> MTTYLEFIQQNEERDGVRFSWNVWPSSRLEATRMVVPV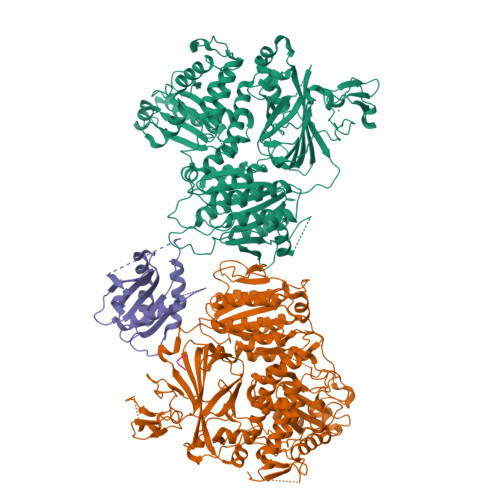AALFTPLKERPDLPPIQYEPVLCSRTTCRAVLNPLCQVDYRAKLWACNFCYQRNQFPPSYAGISELNQPAELLPQFSSIEYVVLRGPQMPLIFLYVVDTCMEDEDLQALKESMQMSLSLLPPTALVGLITFGRMVQVHELGCEGISKSYVFRGTKDLSAKQLQEMLGLSKVPLTQATRGPQVQQPPPSNRFLQPVQKIDMNLTDLLGELQRDPWPVPQGKRPLRSSGVALSIAVGLLECTFPNTGARIMMFIGGPATQGPGMVVGDELKTPIRSWHDIDKDNAKYVKKGTKHFEALANRAATTGHVIDIYACALDQTGLLEMKCCPNLTGGYMVMGDSFNTSLFKQTFQRVFTKDMHGQFKMGFGGTLEIKTSREIKISGAIGPCVSLNSKGPCVSENEIGTGGTCQWKICGLSPTTTLAIYFEVVNQHNAPIPQGGRGAIQFVTQYQHSSGQRRIRVTTIARNWADAQTQIQNIAASFDQEAAAILMARLAIYRAETEEGPDVLRWLDRQLIRLCQKFGEYHKDDPSSFRFSETFSLYPQFMFHLRRSSFLQVFNNSPDESSYYRHHFMRQDLTQSLIMIQPILYAYSFSGPPEPVLLDSSSILADRILLMDTFFQILIYHGETIAQWRKSGYQDMPEYENFRHLLQAPVDDAQEILHSRFPMPRYIDTEHGGSQARFLLSKVNPSQTHNNMYAWGQESGAPILTDDVSLQVFMDHLKKLAVSSA;> EGLRVVNLLQERNMLPSTPLKPPVPNLHEDIQKLNCNPELFRCTLTSIPQTQALLNKAKLPLGLLLHPFKDLVQLPVVTSSTIVRCRSCRTYINPFVSFLDQRRWKCNLCYRVNDVPEEFLYNPLTRVYGEPHRRPEVQNATIEFMAPSEYMLRPPQPPVYLFVFDVSHNAVETGYLNSVCQSLLDNLDLLPGNTRTKIGFITFDSTIHFYGLQESLSQPQMLIVSDIEDVFIPMPENLLVNLNESKELVQDLLKTLPQMFTKTLETQSALGPALQAAFKLMSPTGGRMSVFQTQLPTLGVGALKPREEPNHRSSAKDIHMTPSTDFYKKLALDCSGQQVAVDLFLLSGQYSDLASLGCISRYSAGSVYYYPSYHHQHNPVQVQKLQKELQRYLTRKIGFEAVMRIRCTKGLSIHTFHGNFFVRSTDLLSLPNVNPDAGYAVQMSVEESLTDTQLVSFQSALLYTSSKGERRIRVHTLCLPVVSTLNDVFLGADVQAISGLLANMAVDRSMTASLSDARDALVNAVIDSLSAYRSSVLSNQQPGLMVPFSLRLFPLFVLALLKQKSFQTGTNARLDERIFAMCQVKNQPLVYLMLTTHPSLYRVDNLSDEGALNISDRTIPQPPILQLSVEKLSRDGAFLMDAGSVLMLWVGKNCTQNFLSQVLGVQNYASIPQPMTDLPELDTPESARIIAFISWLREQRPFFPILYVIADESPMKANFLQNMIEDRTESALSYYEFLLHIQQQVNK;> MVLLTMIARVADGLPLAASMQEDEQSGRDLQQYQSQAKQLFRKLNEQSPTRCTLEAGAMTFHYIIEQGVCYLVLCEAAFPKKLAFAYLEDLHSEFDEQHGKKVPTVSRPYSFIEFDTFIQKTKKLYIDSRARRNLGSINTELQDVQRIMVANIEEVL;> SLV> VLLESEQFLTELTRLFQKCRTSGSVYITLKKYDGRTKPIPKKGTVEGFEPADNKCLLRATDGKK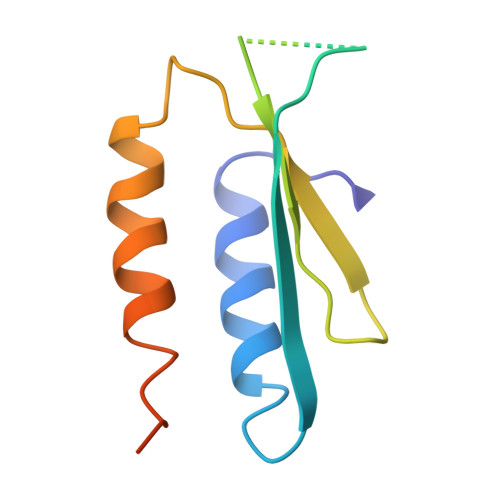KISTVVSSKEVNKFQMAYSNLLRANMDGLKKRDKKNKTKKTK> GAMDPGGGGSSAADPAIPEEVWNIKQMIKLTQEH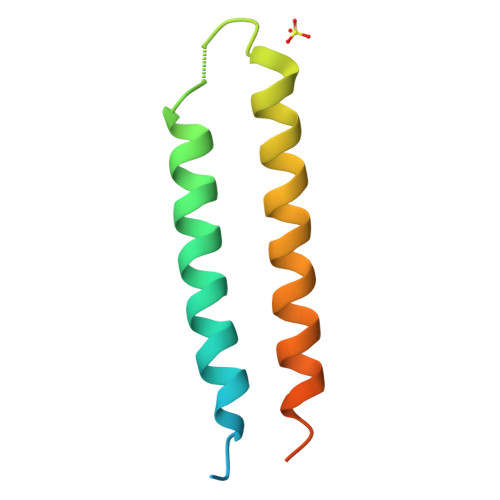IEALLDKFGGEHNPPSIYLEAYEEYTSKLDALQQREQQLLESLGNGTDFSVSSS> NLYQFKNMIQCTVPSRSWADFADYGCYCGKGGSGTPVDDLDRCCQTHDNCYNEAENISGCR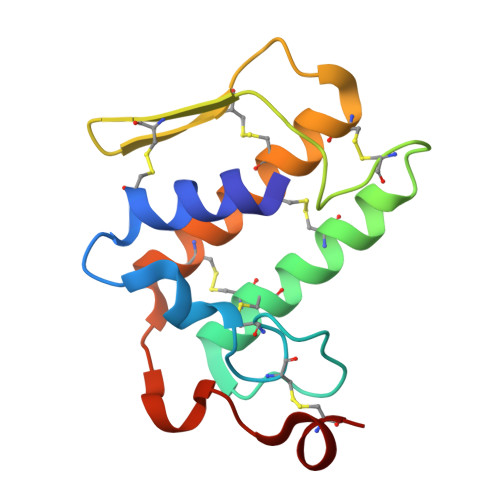PYFKTYSYECTQGTLTCKGDNNACAASVCDCDRLAAICFAGAPYNDDNYNIDLKARCN>MLSHMVLTRQDIGRAASYYEDGADDYYAKDGDASEW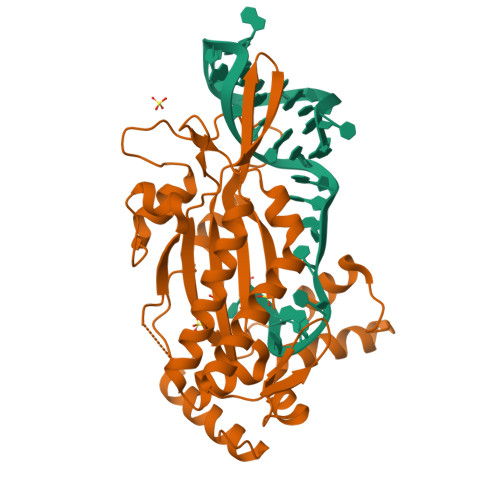QGKGAEELGLSGEVDSKRFRELLAGNIGEGHRIMRSATRQDSKERIGLDLTFSAPKSVSLQALVAGDAEIIKAHDRAVARTLEQAEARAQARQKIQGKTRIETTGNLVIGKFRHETSRERDPQLHTHAVILNMTKRSDGQWRALKNDEIVKATRYLGAVYNAELAHELQKLGYQLRYGKDGNFDLAHIDRQQIEGFSKRTEQIAEWYAARGLDPNSVSLEQKQAAKVLSRAKKTSVDREALRAEWQATAKELGIDFS[2x]>GSHMDYNKRSSVSTVPNAAPIRVGFVGLNAAKGWAIKTHYPAILQLSSQFQITALYSPKIETSIATIQRLKLSNATAFPTLESFASSSTIDMIVIAIQVASHYEVVMPLLEFSKNNPNLKYLFVEWALACSLDQAESIYKAAAERGVQTIISLQGRKSPYILRAKELISQGYIGDINSIEIAGNGGWYGYERPVKSPKYIYEIGNGVDLVTTTFGHTIDILQYMTSSYFSRINAMVFNNIPEQELIDERGNRLGQRVPKTVPDHLLFQGTLLNGNVPVSCSFKGGKPTKKFTKNLVIDIHGTKRDLKLEGDAGFAEISNLVLYYSGTRANDFPLANGQQAPLDPGYDAGKEIMEVYHLRNYNAIVGNIHRLYQSISDFHFNTKKIPELPSQFVMQGFDFEG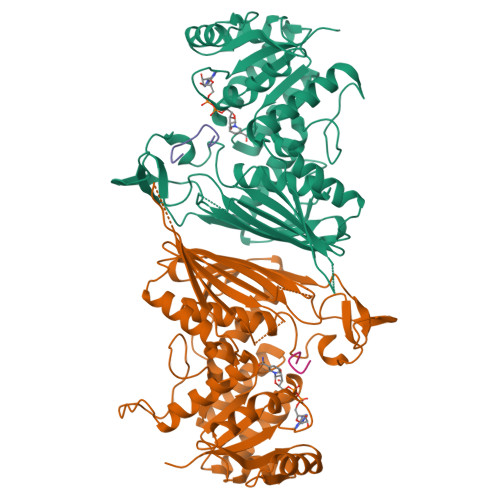FPTLMDALILHRLIESVYKSNMMGSTLNVSNISHYSL[2x];>[2x]GMFNTTTMDDVYNYLFDDEDT>QDSTSDLIPAPPLSKVPLQQNFQDNQFHGKWYVVGEAGNSLLREDKDPRKMYATIYELKEDKSYNVTSVRFRSKKCHYLIRTFVPGSQPGEFTLGLIKSKPGHTSFLVRVVSTNYNQHAMVFFKTVAQNREYFFITLYGRTKELTSELKENFIRFSKSLGLPENHIVFPVPIDQCIDGSAWSHPQFEK[3x];>[3x]PLSPPTNLHLEANPDTGVLTVSWERSTTPDITGYRITTTPTNGQQGNSLEEVVHADQSSCTFDNLSPGLEYNVSVYTVKDDKESVPISDTIIPEVPQLTDLSFVDITDSSIGLRWTPLNSSTIIGYRITVVAAGEGIPIFEDFVDSSVGYYTVTGLEPGIDYDISVITLINGGESAPTTLTQ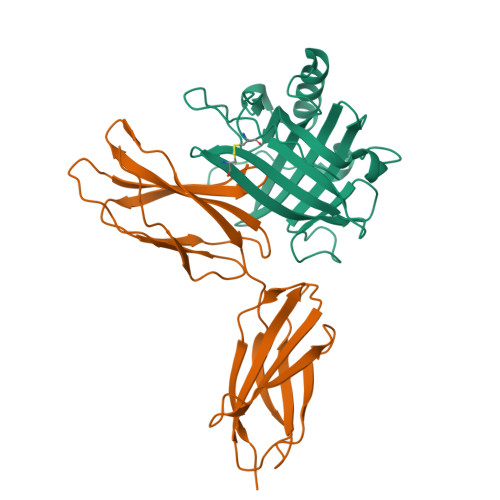QTAVPPPTDLRFTNIGPDTMRVTWAPPPSIDLTNFLVRYSPVKNEEDVAELSISPSDNAVVLTNLLPGTEYVVSVSSVYEQHESTPLRGRQKTGSAHHHHHH3-hexanoyl-4-hydroxy-5-(4-hydroxyphenyl)pyridin-2(1H)-one | C17 H19 N O4 | 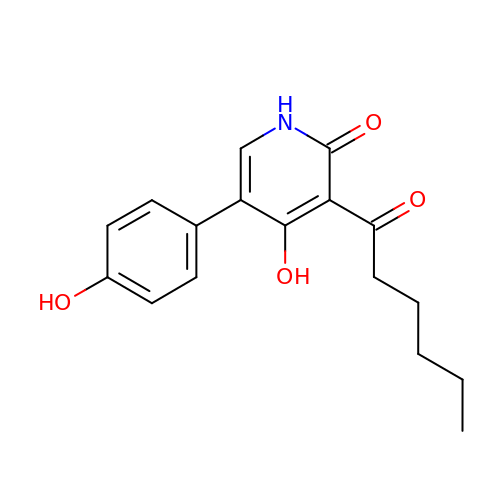NUFZHWWYFUWCIM-UHFFFAOYSA-N>GPLGSMERKISRIHLVSEPSITHFLQVSWEKTLESGFVITLTDGHSAWTGTVSESEISQEADDMAMEKGKYVGELRKALLSGAGPADVYTFNFSKESCYFFFEKNLKDVSFRLGSFNLEKVENPAEVIRELICYCLDTIAENQAK[4x];>GPLGSMEELEQGLLMQPWAWLQLAENSLLAKVFITKQGYALLVSDLQQVWHEQVDTSVVSQRAKELNKRLTAPPAAFLCHLDNLLRPLLKDAAHPSEATFSCDCVADALILRVRSELSGLPFYWNFHCMLAS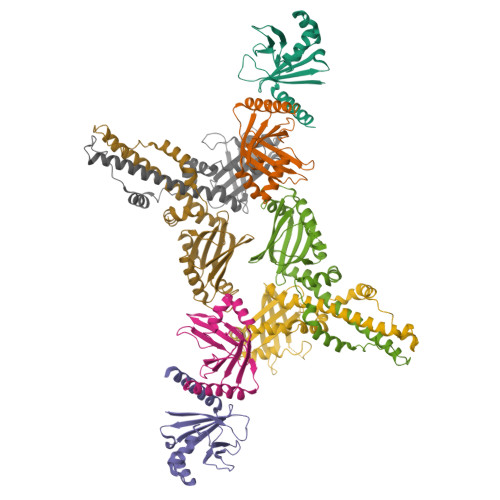PSLVSQHLIRPLMGMSLALQCQVRELATLLHMKDLEIQDYQESGATLIRDRLKTEPFEENSFLEQFMIEKLPEACSIGDGKPFVMNLQDLYMAVTTQ[4x]>[2x]SRAPAPATPHAPDHSPAPNSPTLTRPPEGPKFPRVKNWELGSITYDTLCAQSQQDGPCTPRRCLGSLVLPRKLQTRPSPGPPPAEQLLSQARDFINQYYSSIKRSGSQAHEERLQEVEAEVASTGTYHLRESELVFGAKQAWRNAPRCVGRIQWGKLQVFDARDCSSAQEMFTYICNHIKYATNRGNLRSAITVFPQRAPGRGDFRIWNSQLVRYAGYRQQDGSVRGDPANVEIT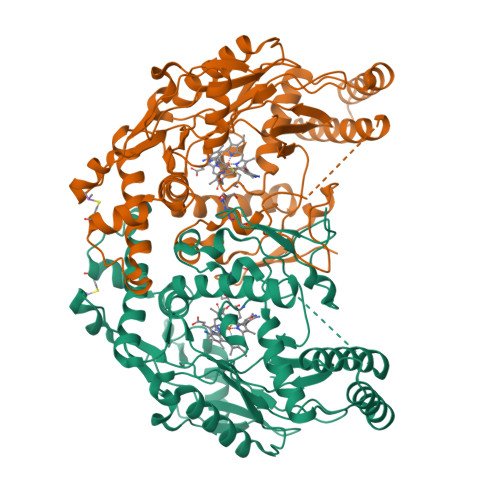ELCIQHGWTPGNGRFDVLPLLLQAPDEAPELFVLPPELVLEVPLEHPTLEWFAALGLRWYALPAVSNMLLEIGGLEFSAAPFSGWYMSTEIGTRNLCDPHRYNILEDVAVCMDLDTRTTSSLWKDKAAVEINLAVLHSFQLAKVTIVDHHAATVSFMKHLDNEQKARGGCPADWAWIVPPISGSLTPVFHQEMVNYILSPAFRYQPDPW>MKQYLELMQKVLDEGTQKNDRTGTGTLSIFGHQMRFNLQDGFPLVTTKRCHLRSIIHELLWFLQGDTNIAYLHENNVTIWDEWADENGDLGPVYGKQWRAWPTPDGRHIDQITTVLNQLKNDPDSRRIIVSAWNVGELDKMALAPCHAFFQFY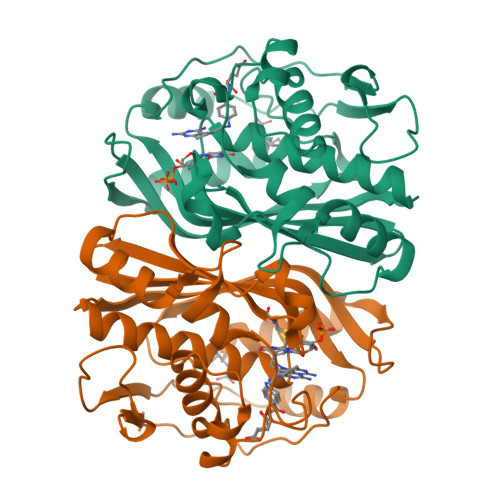VADGKLSCQLYQRSCDVFLGLPFNIASYALLVHMMAQQCDLEVGDFVWTGGDTHLYSNHMDQTHLQLSREPRPLPKLIIKRKPESIFDYRFEDFEIEGYDPHPGIKAPVAI[2x]>GSTGGVQTVTLIPGDGIGPEISAAVMKIFDAAKAPIQWEERNVTAIQGPGGKWMIPSEAKESMDKNKMGLKGPLKTPIAAGHPSMNLLLRKTFDLYANVRPCVSIEGYKTPYTDVNIVTIRENTEGEYSGIEHVIVDGVVQSIKLITEGASKRIAEFAFEYARNNHRSNVTAVHKANIMRMSDGLFLQKCREVAESCKDIKFNEMYLDTVCLNMVQDPSQFDVLVMPNLYGDILSDLCAGLIGGLGVTPSGNIGANGVAIFESVHGTAPDIAGKDMANPTALLLSAVMMLRHMGLFDHAARIEAACFATIKDGKSLTKDLGGNAKCSDFTEEICRRVKDLD[8x];>ASRSQAEDVRVEGSFPVTMLPGDGVGPELMHAVKEVFKAAAVPVEFQEHHLSEVQNMASEEKLEQVLSSMKENKVAIIGKIHTPMEYKGELASYDMRLRRKLDLFANVVHVKSLPGYMTRHNNLDLVIIREQTEGEYSSLEHESARGVIECLKIVTRAKSQRIAKFAFDYATKKGRGKVTAVHKANIMKLGDGLFLQCCEEVAELYPKIKFETMIIDNCCMQLVQNPYQFDVLVMPNLYGNIIDNLAAGLVGGAGVVPGESYSAEYAVFETGARHPFAQAVGRNIANPTAMLLSASNMLRHLNLEYHSSMIADAVKKVIKVGKVRTSDMGGYATCHDFTEEICRRVKDLDENL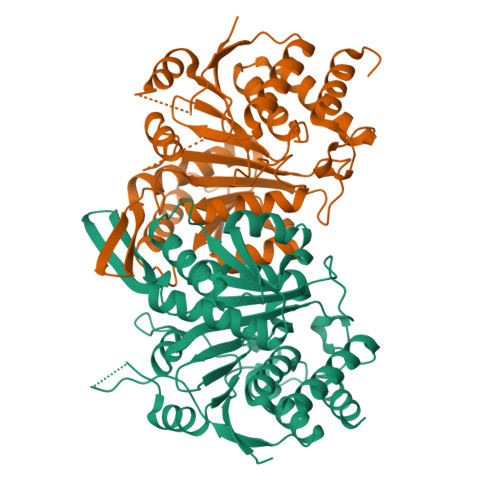YFQ[8x]>[2x]XELENIVANTVLLKAREGGGGNRKGKSKKWRQMLQFPHISQCEELRLSLERDY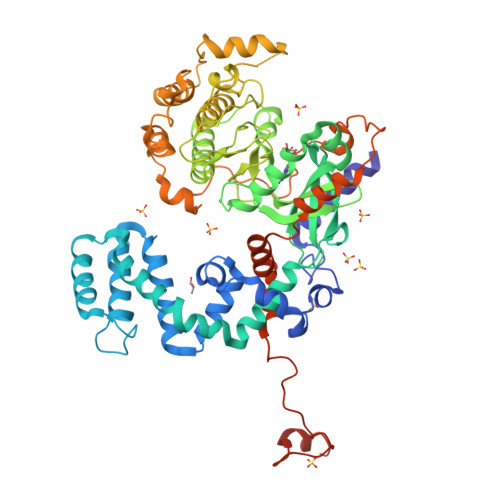HSLCERQPIGRLLFREFCATRPELSRCVAFLDGVAEYEVTPDDKRKACGRQLTQNFLSHTGPDLIPEVPRQLVTNCTQRLEQGPCKDLFQELTRLTHEYLSVAPFADYLDSIYFNRFLQWKWLERQPVTKNTFRQYRVLGKGGFGEVCACQVRATGKMYACKKLEKKRIKKRKGEAMALNEKQILEKVNSRFVVSLAYAYETKDALCLVLTLMNGGDLKFHIYHMGQAGFPEARAVFYAAEICCGLEDLHRERIVYRDLKPENILLDDHGHIRISDLGLAVHVPEGQTIKGRVGTVGYMAPEVVKNERYTFSPDWWALGCLLYEMIAGQSPFQQRKKKIKREEVERLVKEVPEEYSERFSPQARSLCSQLLCKDPAERLGCRGGSAREVKEHPLFKKLNFKRLGAGMLEPPFKPDPQAIYCKDVLDIEQFSTVKGVELEPTDQDFYQKFATGSVPIPWQNEMVETECFQELNVFGLDGSVPPDLDWKGQPPAPPKKGLLQRLFSRQDCCGNCSDSEEELPTRL>MDLTSKVNRLLAEFAGRIGLPSLSLDEEGMASLLFDEQVGVTLLLLAERERLLLEADVVGIDVLGEGIFRQLASFNRHWHRFDLHFGFDELTGKVQLYAQILAAQLTLECFEATLANLLDHAEFWQRLLPCAS[12x];>GTEAVGHFEGRSVTRAAVRGEDRSSVAGLARWLARNVAGDPRSEQALQRLA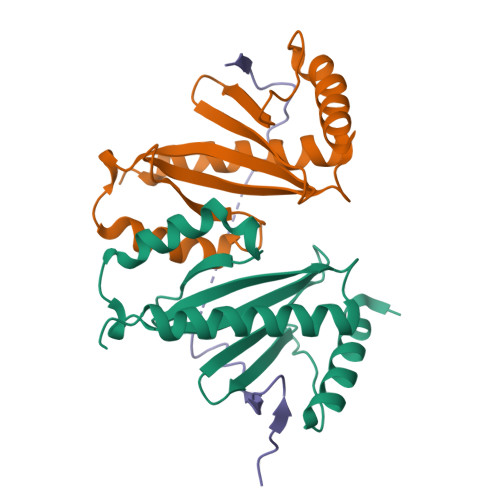DGDGTPLEARTVRRR[6x]> GSHMAVHLTRIYTRTGDDGTTGLSDMSRVAKTDARLVAYADCDEANAAIGAALALGHPDTQITDVLRQIQNDLFDAGADLSTPIVENPKHPPLRIAQSYIDRLEGWCDA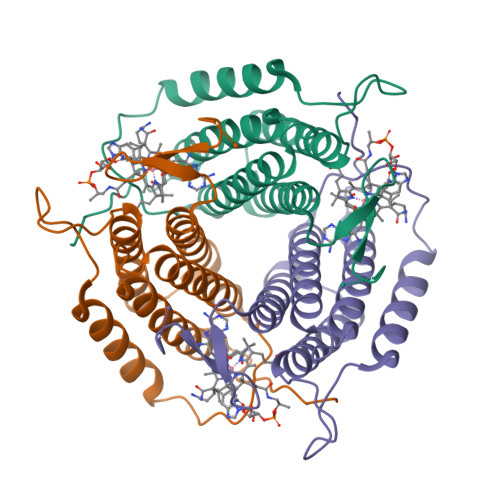YNAGLPALKSFVLPGGSPLSALLHVARTVVRRAERSAWAAVDAHPEGVSVLPAKYLNRLSDLLFILSRVANPDGDVLWRPGGDRTAS>[4x]LVSSPSTLNPGTNVAKLAEQAPVHWVSVAQIENSLTGRPPMAVGFDIDDTVLFSSPGFWRGKKTYSPDSDDYLKNPAFWEKMNNGWDEFSIPKEAARQLIDMHVRRGDSIYFV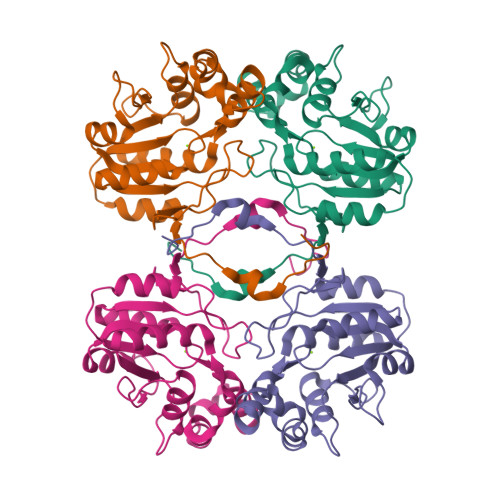TGRSQTKTETVSKTLADNFHIPAANMNPVIFAGDKPEQNTRVQWLQEKNMRIFYGDSDNDITAARDCGIRGIRILRAANSTYKPLPQAGAFGEEVIVNSEY> GMDIQNMPREQLGVCAEGNLHSVYLMFNANDNVESQLRPCIANVAQYIYELTDQYSDSAFNGFVAIGANYWDSLYPESRPEMLKPFPAMQEG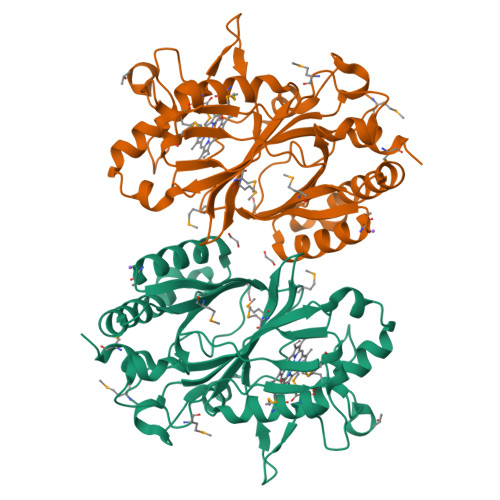NREAPAIEYDLFVHLRCDRYDILHLVANEISQMFEDLVELVEEERGFRFMDSRDLTGFVDGTENPKGRHRQEVALVGSEDPEFKGGSYIHVQKYAHNLSKWHRLPLKKQEDIIGRTKQDNIEYESEDKPLTSHIKRVNLKDENGKSIEILRQSMPYGSLKEQGLMFISTCRTPDHFEKMLHSMVFGDGAGNHDHLMHFTSALTGSSFFAPSLDFLMQFDN>[2x]NLKPVDAMQCFDCHTQIEDMHTVGKHATVNCVHCHDATEHVETASSRRMGERPVTRMDLEACATCHTAQFNSFVEVR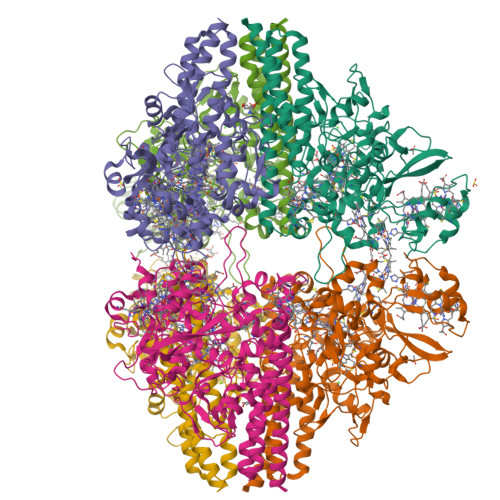HESHPRLEKATPTSRSPMFDKLIAGHGFAFEHAEPRSHAFMLVDHFVVDRAYGGRFQFKNWQKVTDGMGAVRGAWTVLTDADPESSDQRRFLSQTATAANPVCLNCKTQDHILDWAYMGDEHEAAKWSRTSEVVEFARDLNHPLNCFMCHDPHSAGPRVVRDGLINAVVDRGLGTYPHDPVKSEQQGMTKVTFQRGREDFRAIGLLDTADSNVMCAQCHVEYNCNPGYQLSDGSRVGMDDRRANHFFWANVFDYKEAAQEIDFFDFRHATTGAALPKLQHPEAETFWGSVHERNGVACADCHMPKVQLENGKVYTSHSQRTPRDMMGQACLNCHAEWTEDQALYAIDYIKNYTHGKIVKSEYWLAKMIDLFPVAKRAGVSEDVLNQARELHYDAHLYWEWWTAENSVGFHNPDQARESLMTSISKSKEAVSLLNDAIDAQVASR>TTTEVVMENVTAFWEEGGTPVLKDINFKIERGQLLAVAGSTGAGKTSLLMVIMGELEPSEGKIKHSGRISFCSQFSWIMPGTIKENIIGDSYDEYRYRSVIKACQLEEDISKFAEKDNIVLGEGGITLSGGQRARISLARAVYKDADLYLLDSPFGYLDVLTEKEIFESCVCKLMANKTRILVTSKMEHLKKA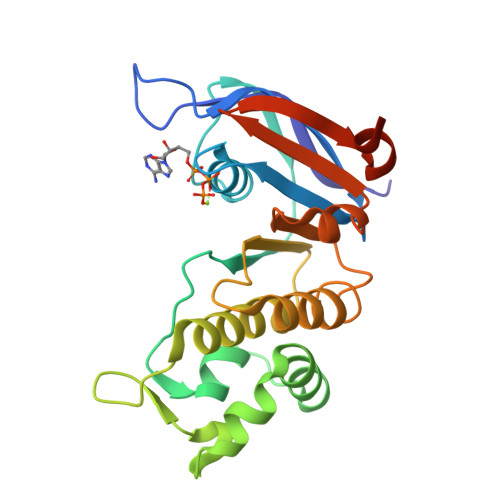DKILILHEGSSYFYGTFSELQNLQPDFSSKLMG[2x]7-amino-2-tert-butyl-4-{[2-(1H-imidazol-4-yl)ethyl]amino}pyrido[2,3-d]pyrimidine-6-carboxamide | C17 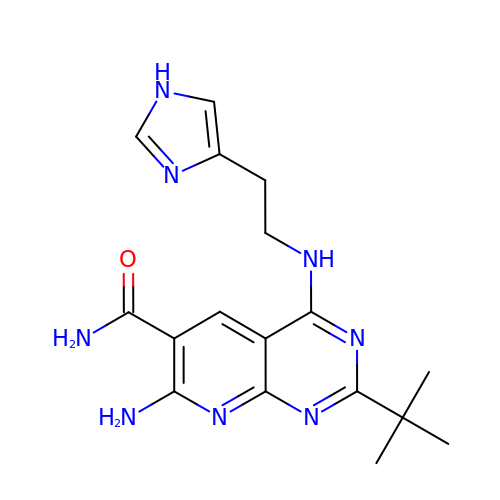H22 N8 O | XESUNWBIAADLPI-UHFFFAOYSA-N> SIVLEPIYWNSSNSKFLPGQGLVLYPQIGDKLDIICPKVDSKTVGQYEYYKVYMVDKDQADRCTIKKENTPLLNCARPDQDVKFTIKFQEFSPNLWGLEFQKNKDYYIISTSNGSLEGLDNQEGGVCQTRAMKILMKVGQDASSAGSARNHGPTRR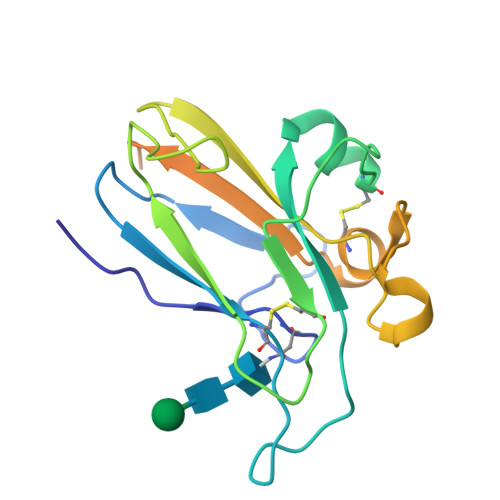PELEAGTNGRSSTTSPFVKPNP> TVPSIVLNDGNSIPQLGYGVFKVPPADTQRAVEEALEVGYRHIDTAAIYGNEEGVGAAIAASGIARDDLFITTKLWNDRHDGDEPAAAIAESLAKLALDQVDLYLVHWPTPAADNYVHAWEKMIELRAAG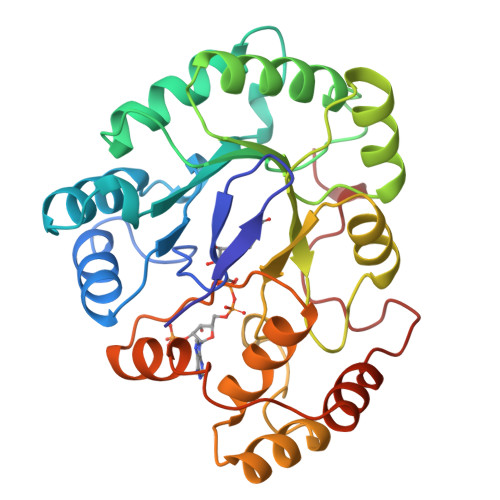LTRSIGVSNHLVPHLERIVAATGVVPAVNQIELHPAYQQREITDWAAAHDVKIESWGPLGQGKYDLFGAEPVTAAAAAHGKTPAQAVLRWHLQKGFVVFPKSVRRERLEENLDVFDFDLTDTEIAAIDAMDPGDGSGRVSAHPDEVD> GFAN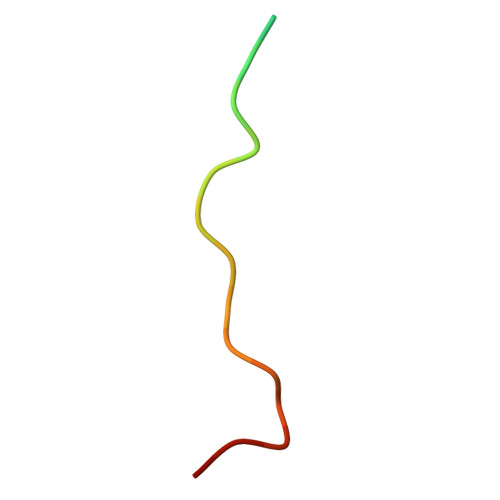RFSKPKGPRNPPPTWNI>MAAPKGNRFWEARSSHGRNPKFESPEALWAACCEYFEWVEA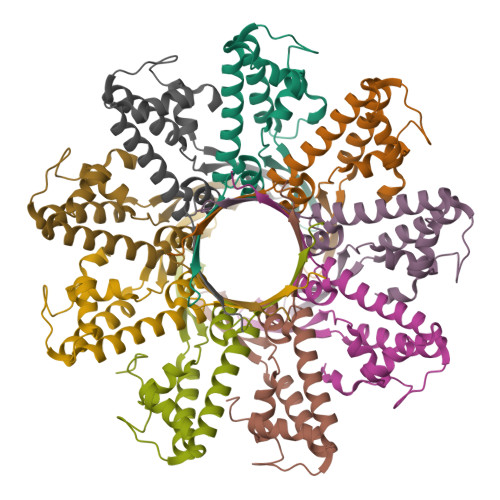NPLWEMKAFSYQGEVIQEPIAKMRAMTITGLTLFIDVTLETWRTYRLREDLSEVVTRAEQVIYDQKFSGAAADLLNANIIARDLGLKEQSQVEDVTPDKGDRDKRRSRIKELFNRGTGRDS[9x]>RSNESTSIRVAVEKVDQLINLVGELVITQSMLAQRSSELDPVNHGDLITSMGQLQRNARDLQESVMSIRMMPMEYVFSRYPRLVRDLAGKLGKQVELTLVGSSTEL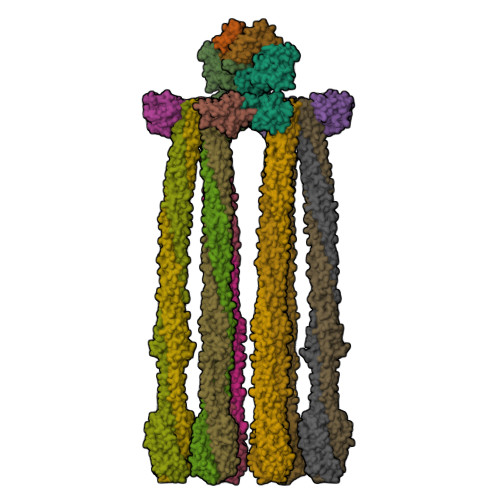DKSLIERIIDPLTHLVRNSLDHGIELPEKRLAAGKNSVGNLILSAEHQGGNICIEVTDDGAGLNRERILAKAASQGLTVSENMSDDEVAMLIFAPGFSTAEQVTDVSGRGVGMDVVKRNIQKMGGHVEIQSKQGTGTTIRILLPLTLAILDGMSVRVADEVFILPLNAVMESLQPREADLHPLAGGERVLEVRGEYLPIVELWKVFNVAGAKTEATQGIVVILQSGGRRYALLVDQLIGQHQVVVKNLESNYRKVPGISAATILGDGSVALIVDVSALQAINREQ[2x];>[2x]MSMDISDFYQTFFDEADELLADMEQHLLVLQPEAPDAEQLNAIFRAAHSIKGGAGTFGFSVLQETTHLMENLLDEARRGEMQLNTDIINLFLETKDIMQEQLDAYKQSQEPDAASFDYICQALRQLALEAK;>SGQEFLVFTLGDEEYGIDILKVQEIRGYDQVTRIANTPAFIKGVTNLRGVIVPIVDLRIKFSQVDVDYNDNTVVIVLNLGQRVVGIVVDGVSDVLSLTAEQIRPAPEFAVTLSTEYLTGLGALGDRMLILVNIEKLLNSEEMA[4x];>MLKRIKIVTSLLLVLAVFGLLQLTSGGLFFNALKNDKENFTVLQTIRQQQSTLNGSWVALLQTRNTLNRAGIRYMMDQNNIGSGSTVAELMESASISLKQAEKNWADYEALPRDPRQSTAAAAEIKRNYDIYHNALAELIQLLGAGKINEFFDQPTQGYQDGFEKQYVAYMEQNDRLHDIAVSDNNASYSQAMWILVGVMIVVLAVIFAVWFGIKASLVAPMNRLIDSIRHIAGGDLVKPIEVDGSNEMGQLAESLRHMQGELMRTVGDVRNGANAIYSGASEIATGNNDLSSRTEQQAASLEETAASMEQLTATVKQNAENARQASHLALSASETAQRGGKVVDNVVQTMRDISTSSQKIADIISVIDGIAFQTNILALNAAVEAARAGEQGRGFAVVAGEVRNLAQRSAQAAREIKSLIEDSVGKVDVGSTLVESAGETMAEIVSAVTRVTDIMGEIASASDEQSRGIDQVGLAVAEMDRVTQQNAALVEESAAAAAALEEQASRLTEAVAVFR[12x]>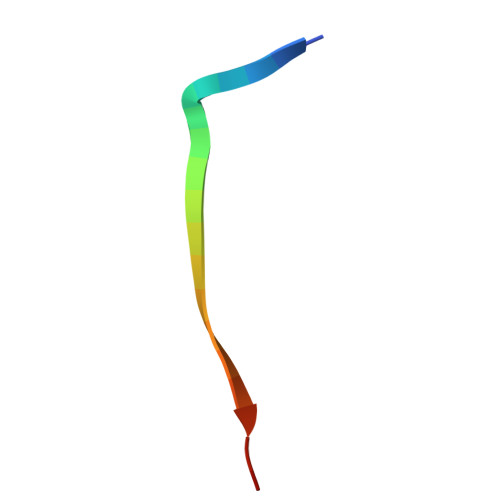 GSFLPNSEQQKSADIVFSSP> PEKVTVVP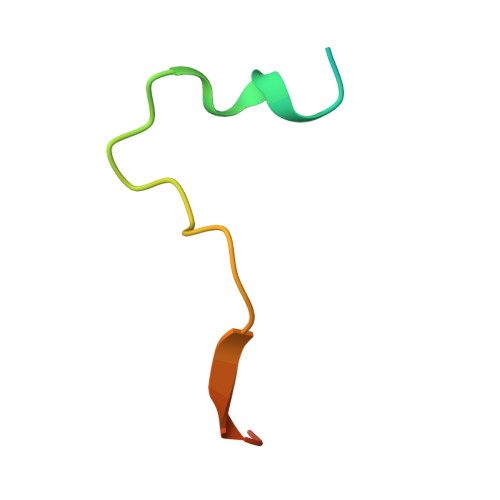KFGDWDENNPSSADGYTHIFNKVREER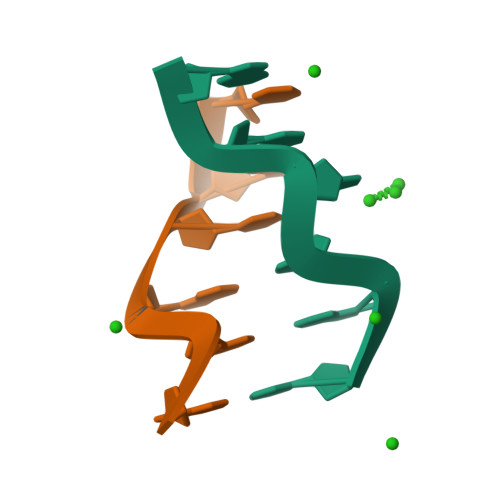>[8x]CGCGCG> PIETVPVKLKPGMDGPKVKQWPLTEEKIKALVEICTEMEKEGKISKIGPENPYNTPVFAIKKKDSTKWRKLVDFRELNKRTQDFWEVQLGIPHPAGLKKKKSVTVLDVGDAYFSVPLDEDFRKYTAFTIPSINNETPGIRYQYNVLPQGWKGSPAIFQSSMTKILEPFRKQNPDIVIYQYMDDLYVGS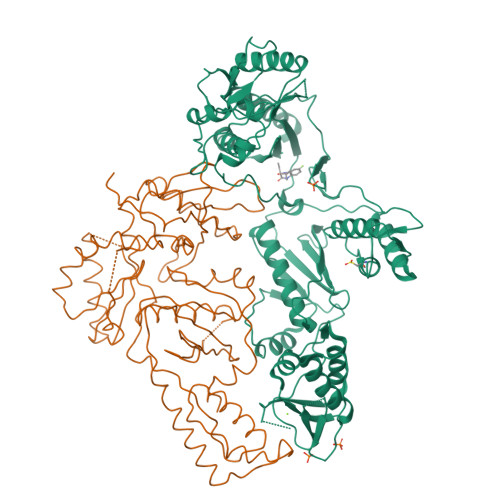DLEIGQHRTKIEELRQHLLRWGLTTPDKKHQKEPPFLWMGYELHPDKWTVQPIVLPEKDSWTVNDIQKLVGKLNWASQIYPGIKVRQLCKLLRGTKALTEVIPLTEEAELELAENREILKEPVHGVYYDPSKDLIAEIQKQGQGQWTYQIYQEPFKNLKTGKYARMRGAHTNDVKQLTEAVQKITTESIVIWGKTPKFKLPIQKETWETWWTEYWQATWIPEWEFVNTPPLVKLWYQLEKEPIVGAETFYVDGAANRETKLGKAGYVTNRGRQKVVTLTDTTNQKTELQAIYLALQDSGLEVNIVTDSQYALGIIQAQPDQSESELVNQIIEQLIKKEKVYLAWVPAHKGIGGN;> IETVPVKLKPGMDGPKVKQWPLTEEKIKALVEICTEMEKEGKISKIGPENPYNTPVFAIKKKDSTKWRKLVDFRELNKRTQDFWEVQLGIPHPAGLKKKKSVTVLDVGDAYFSVPLDEDFRKYTAFTIPSINNETPGIRYQYNVLPQGWKGSPAIFQSSMTKILEPFRKQNPDIVIYQYMDDLYVGSDLEIGQHRTKIEELRQHLLRWGLTTPDKKHQKEPPFLWMGYELHPDKWTVQPIVLPEKDSWTVNDIQKLVGKLNWASQIYPGIKVRQLCKLLRGTKALTEVIPLTEEAELELAENREILKEPVHGVYYDPSKDLIAEIQKQGQGQWTYQIYQEPFKNLKTGKYARMRGAHTNDVKQLTEAVQKITTESIVIWGKTPKFKLPIQKETWETWWTEYWQATWIPEWEFVNTPPLVKLWYQLEK>[12x]TTIVSVRRNGHVVIAGDGQATLGNTVMKGNVKKVRRLYNDKVIAGFAGGTADAFTLF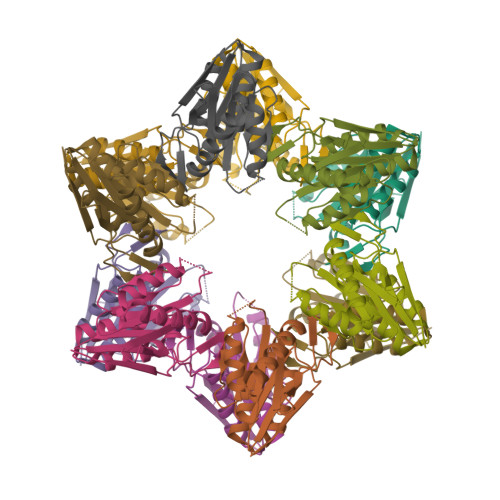ELFERKLEMHQGHLVKAAVELAKDWRTDRMARKLEALLAVADETASLIITGNGDVVQPENDLIAIGSGGPYAQAAARALLENTELSAREIAEKALDIAGDICIYTNHFHTIEELSYK> MDEQ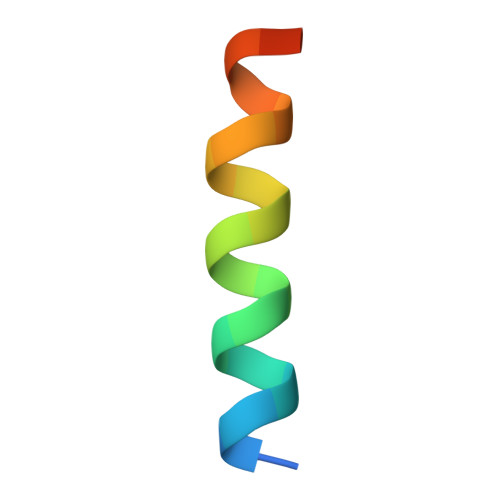EALNSIMNDLVALQMNRR>[2x]NKRTTVNILYVRKPDEFYVTLPHFQKAINNLQKSVQKAAAAMYQNMLPRTDWQVGDMCYARVQANCDSQALWYRGVVTGVIPPGI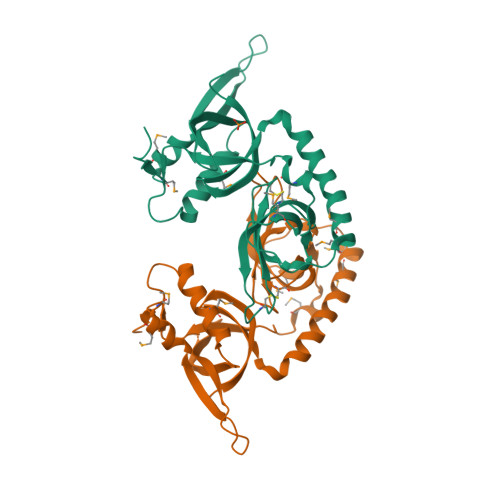TCPIVRYQVHLRDLGELIDDVHSSSLANIDEADMRISSSAKRCHLHGIRPIGDEWSKDAIDFFMDQLKAYNEIHVTGRGRTENSLSVILWGSLSILTGPFSPATIKYVNINKALLMAGMAEKDHNSD> EIV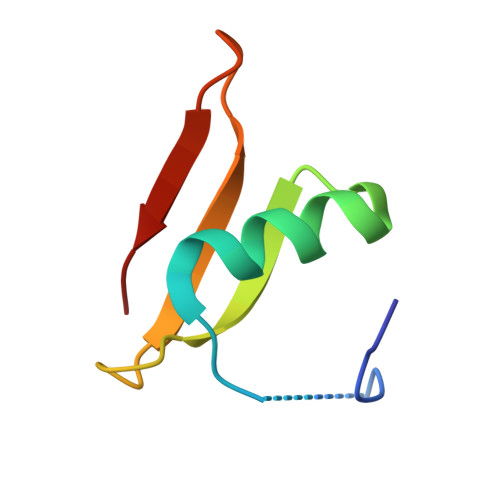RTKQFSLKPMDSEEAVLQMNLLGHSFYVYTDAETNGTNIVYSRKDGKYGLIETN> GPGSSLQTSDVVIHRKENEGFGFVIISSLNRPESGATITVPH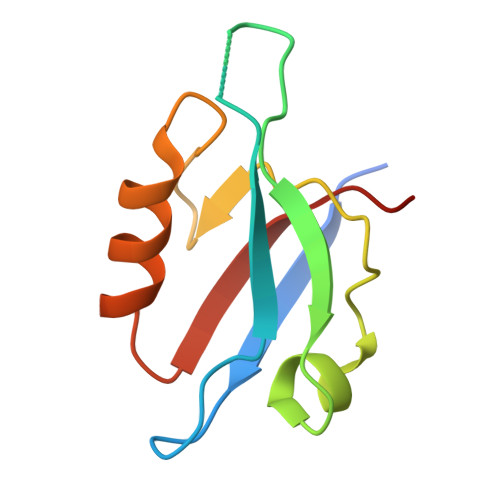KIGRIIDGSPADRCAKLKVGDRILAVNGQSIINMPHADIVKLIKDAGLSVTLRIIPQEE>GPSFWLGNETLKVPLALFALNRQRLCERLRKNPAVQAGSIVVLQGGEETQRYCTDTGVLFRQESFFHWAFGVTEPGCYGVIDVDTGKSTLFVPRLPASHATWMGKIHSKEHFKEKYAVDDVQYVDEIASVLTSQKPSVLLTLRGVNTDSGSVCREASFDGISKFEVNNTILHPEIVECRVFKTDMELEVLRYTNKISSEAHREVMKAVKVGMKEYELESLFEHYCYSRGGMRHSSYTCICGSGENSAVLHYGHAGAPNDRTIQNGDMCLFDMGGEYYCFASDITCSFPANGKFTADQKAVYEAVLRS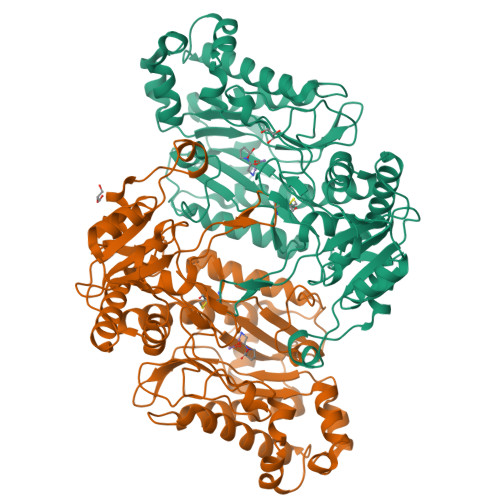SRAVMGAMKPGVWWPDMHRLADRIHLEELAHMGILSGSVDAMVQAHLGAVFMPHGLGHFLGIDVHDVGGYPEGVERIDEPGLRSLRTARHLQPGMVLTVEPGIYFIDHLLDEALADPARASFLNREVLQRFRGFGGVRIEDVVVTDSGIELLTCVPRTVEEIEACMAGCDK[2x]> MFENITAAPADPILGLADLFRADERPGKINLGIGFYKDETGKTPVLTSVKKAEQYLLENETTKNYLGIDGIPEFGRCTQELLFGKGSALINDKRARTAQTPGGTGALRVAADFLAKNTSVKRVWVSNPSWPNHKSVFNSAGLEVREYAYYDAENHTL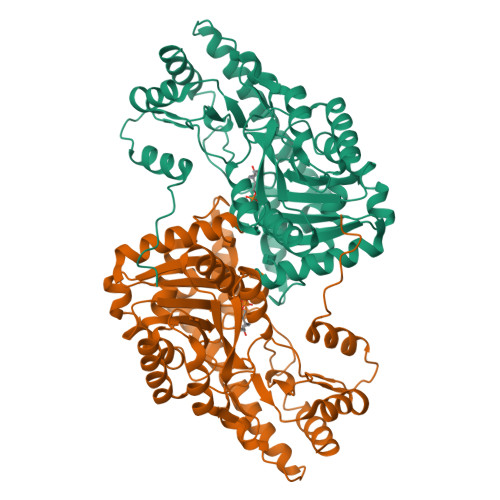DFDALINSLNEAQAGDVVLFHGCCHNPTGIDPTLEQWQTLAQLSVEKGWLPLFDFAYQGFARGLEEDAEGLRAFAAMHKELIVASSYSKNFGLYNERVGACTLVAADSETVDRAFSQMKAAIRANYSNPPAHGASVVATILSNDALRAIWEQELTDMRQRIQRMRQLFVNTLQEKGANRDFSFIIKQNGMFSFSGLTKEQVLRLREEFGVYAVASGRVNVAGMTPDNMAPLCEAIVAVL Hypothesizing that a serpin reflecting a highly conserved sequence may offer insight into the delicate balance between folding and function, we designed conserpin (consensus serpin). To design conserpin we used the consensus approach and a previously reported MSA of 219 serpin sequences. Conserpin (396 aa) shares the highest similarity with α1-AT (137 residue differences; 62% sequence identity). Characterization of its function, structure and folding reveal a serpin that is inhibitory, folds reversibly, is thermostable and resistant to polymerisation.

In order to investigate the effects of a highly destabilizing mutation on conserpin, we introduced E342K313 into conserpin to produce Z-conserpin. Z-conserpin expressed well as a soluble monomer in E. coli, which has not been possible with Z α1-AT7683. Z-conserpin showed a highly similar inhibitory profile to conserpin, with an SI of 2.3 and a kass of 2.1 × 107 M−1 s−1. Z-conserpin exhibits reversible, two-state folding upon chemical denaturation. The equilibrium unfolding and refolding curves overlay almost perfectly, revealing a midpoint of denaturation, [D]50 to be 2.51 ± 0.01 M, an equilibrium m-value, mD-N, of 5.18 kcal mol−1 M−1, and a stability ∆GD-N, of −12.8 kcal mol−1 (a loss of −10.04 kcal mol−1). We therefore repeated equilibrium unfolding using bis-ANS fluorescence, detecting a fluorescent peak at ~2.5 M GuHCl, that is slightly broader and more intense than observed in conserpin, indicating an increase in the intermediate ensemble population, but still smaller than in α1-AT. Native PAGE shows conserpin to remain monomeric except when heated to 90 °C for 10 minutes, whilst Z-conserpin has a complete loss of monomer at 80 °C and forms a slightly higher molecular weight species when heated to 70 °C for 10 minutes. The crystal structure of native Z-conserpin reveals almost no structural differences upon mutation (backbone RMSD = 0.23 Å); the sole differences surrounding E342K313 are small side-chain shifts of K342313 and K290262, most likely as a result of electrostatic repulsion. A caveat is one local residue difference, K343E314, in conserpin that may partially negate the effects of E342K313, due to its salt bridge with K165conserpin. Regardless, the structure of Z-conserpin reveals essentially no structural changes to the native state which disagrees with reports of structural perturbations within the native state808284; therefore favoring the mechanism of Z-variant polymerization via a folding intermediate.

>[2x]MHHHHHHENLYFQGAASSHKLAEANTDFAFSLYRELAKSSPDKNIFFSPVSISSALAMLSLGAKGDTHTQILEGLGFNSEADIHQGFQHLLQTLNRPKGLQLKTANGLFVDKSLKLLDSFLEDSKKLYQAEAFSVDFDPEEAKKQINDWVEKQTNGKIKDLLKDLDSDTVLVLVNAIYFKGKWKKPFDPENTKEEDFHVDEKTTVKVPMMSQKGKFYYYHDDELSCKVLELPYKGNASMLIILPDEGGLQHLEQSLTPETLSKWLKSLTRRSVELYLPKFKIEGTYDLKEVLSNLGITDLFSPGADLSGITEEKLYVSKAVHKAVLEVNKEGTEAAAATGVEIVPRSPPEFKADRPFLFLIRENKTGSILFMGKVVNP> MSGDENPASKPTPVQDVQGDGRWMSLHHRFVADSKDKEPEVVFIGDSLVQLMHQCEIWR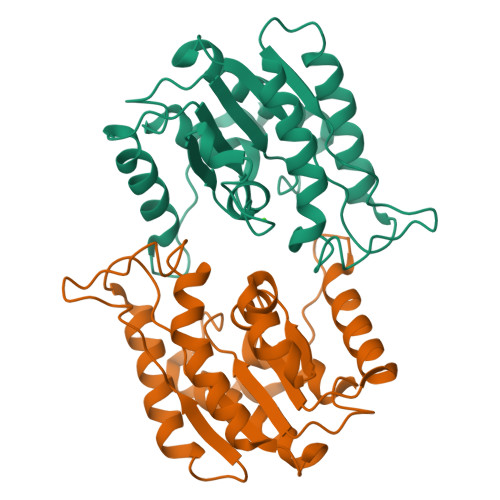ELFSPLHALNFGIGGDSTQHVLWRLENGELEHIRPKIVVVWVGTNNHGHTAEQVTGGIKAIVQLVNERQPQARVVVLGLLPRGQHPNPLREKNRRVNELVRAALAGHPRAHFLDADPGFVHSDGTISHHDMYDYLHLSRLGYTPVCRALHSLLLRLLTQDQGQGGAPLPEPSP;> MSQGDSNPAAIPHAAEDIQGDDRWMSQHNRFVLDCKDKEPDVLFVGDSMVQLMQQYEIWRELFSPLHALNFGIGGDTTRHVLWRLKNGELENIKPKVIVVWVGTNNHENTAEEVAGGIEAIVQLINTRQPQAKIIVLGLLPRGEKPNPLRQKNAKVNQLLKVSLPKLANVQLLDTDGGFVHSDGAISCHDMFDFLHLTGGGYAKICKPLHELIMQLLEETPEEKQTTIA> SDKIIHLTDDSFDTDVLKADGAILVDFWAEWC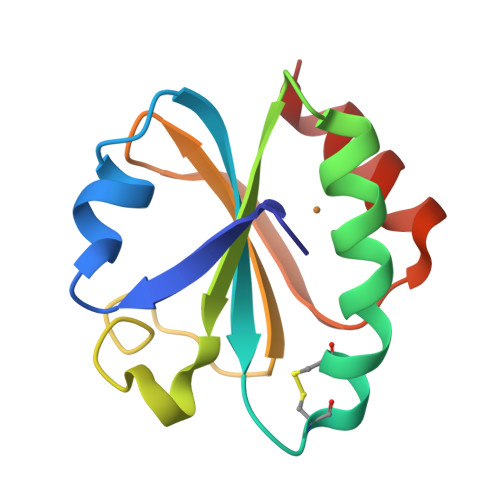GPCEMIAPILDEIADEYQGKLTVAKLNIDQNPGTAPKYGIRGIPTLLLFKNGEVAATKVGALSKGQLKEFLDANLA> TSQKHRDFVAEPMGEKPVGSLAGIGEVLGKKLEERGFDKAYVVLGQFLVLKKDED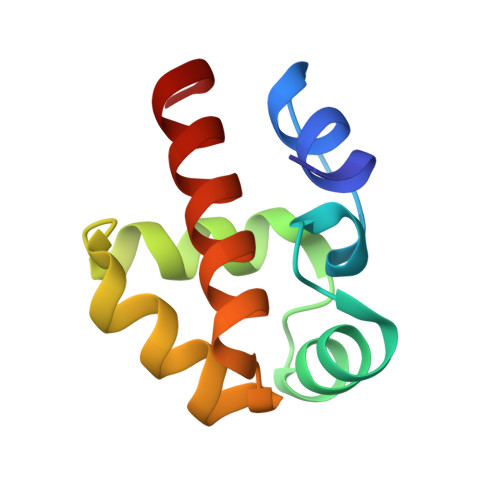LFREWLKDTAGANAKQSRDAFGALREWADAFL> MGINGQQYYIDPTTGQPRKNFLLQNGNDWIYFDKDTGAGTNALKLQFDKGTISADEQYRRGNEAYSYDDKSIENVNGYLTADTWYRPKQILKDGTTWTDSKETDMRPILMVWWPNTVTQAYYLNYMKQYGNLLPASLPSFSTDADSAELNHYSELVQQNIEKRISETGSTDWLRTLMHEFVTKNSMWNKDSENVDYGGLQLQGGFLKYVNSDLTKYANSDWRLMNRTATNIDGKNYGGAEFLLANDIDNSNPVVQAEELNWLYYLMNFGTITGNNPEANFDGIRVNAVDNVDVDLLSIARDYFNAAYNMEQSDASANKHINILEDWGWDDPAYVNKIGNPQLTMDDRLRNAIMDTLSGAPDKNQALNKLITQSLVNRANDNT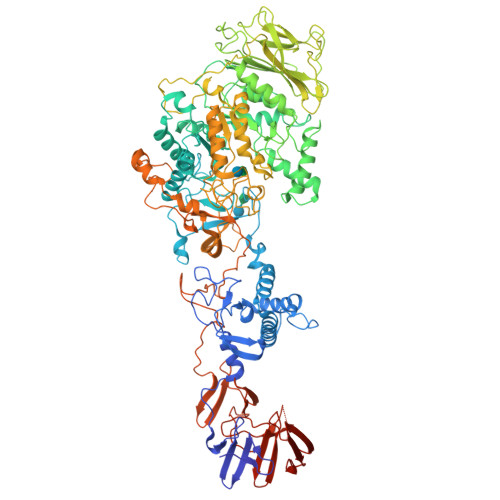ENAVIPSYNFVRAHDSNAQDQIRQAIQAATGKPYGEFNLDDEKKGMEAYINDQNSTNKKWNLYNMPSAYTILLTNKDSVPRVYYGDLYQDGGQYMEHKTRYFDTITNLLKTRVKYVAGGQTMSVDKNGILTNVRFGKGAMNATDTGTDETRTEGIGVVISNNTNLKLNDGESVVLHMGAAHKNQKYRAVILTTEDGVKNYTNDTDAPVAYTDANGDLHFTNTNLDGQQYTAVRGYANPDVTGYLAVWVPAGAADDQDARTAPSDEAHTTKTAYRSNAALDSNVIYEGFSNFIYWPTTESERTNVRIAQNADLFKSWGITTFELAPQYNSSKDGTFLDSIIDNGYAFTDRYDLGMSTPNKYGSDEDLRNALQALHKAGLQAIADWVPDQIYNLPGKEAVTVTRSDDHGTTWEVSPIKNVVYITNTIGGGEYQKKYGGEFLDTLQKEYPQLFSQVYPVTQTTIDPSVKIKEWSAKYFNGTNILHRGAGYVLRSNDGKYYNLGTSTQQFLPSQLSVQDNEGYGFVKEGNNYHYYDENKQMVKDAFIQDSVGNWYYLDKNGNMVANQSPVEISSNGASGTYLFLNNGTSFRSGLVKTDAGTYYYDGDGRMVRNQTVSDGAMTYVLDENGKLVSESFDSSATEAHPLKPGDLNGQKHHHHHH> MYATMESVRLQSEAQQLAEMILQSETAENYRNCYKRLQEDEEAGRIIRSFIKIKEQYEDVQRFGKYHPDYREISRKMREIKRELDLNDKVADFKRAENELQ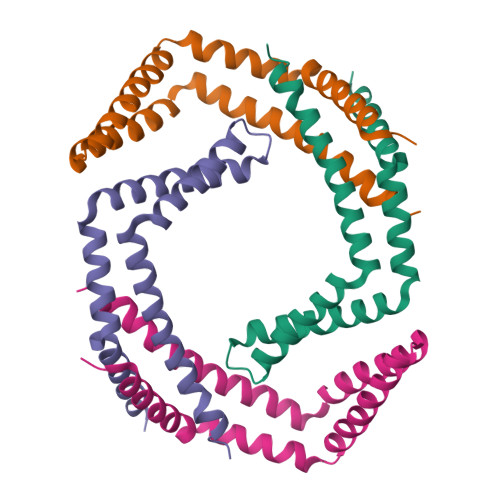SILDEVSVEIGTAVSEHVKV;> GPMTLYSKKDIVQQARNLAKMISETEEVDFFKRAEAQINENDKVSTIVNQIKALQKQAVNLKHYEKHEALKQVEAKIDALQEELEEIPVIQEFRDSQMEVNDLLQLVAHTISNQVTNEIITSTG4-[(9-{4-[(E)-2-cyanoethenyl]-2,6-dimethylphenyl}-8-oxo-8,9-dihydro-7H-purin-2-yl)amino]benzonitrile 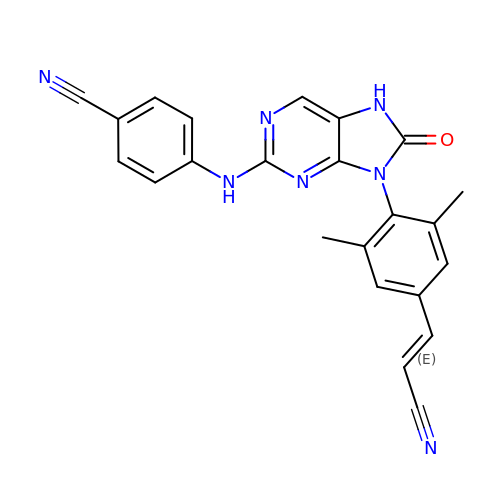| C23 H17 N7 O | NSCZUKITHKGKLS-ONEGZZNKSA-N>[4x]STPSIVIASAARTAVGSFNGAFANTPAHELGATVISAVLERAGVAAGEVNEVILGQVLPAGEGQNPARQAAMKAGVPQEATAWGMNQLCGSGLRAVALGMQQIATGDASI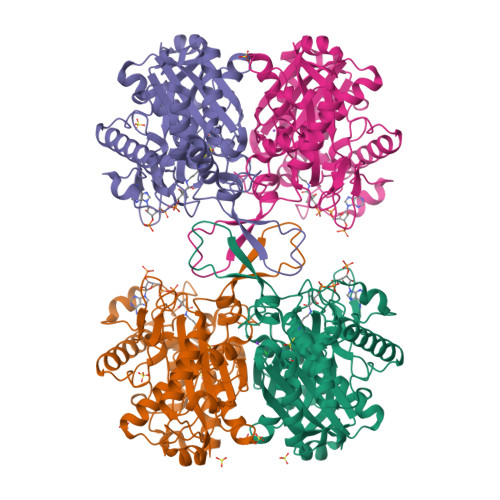IVAGGMESMSMAPHCAHLRGGVKMGDFKMIDTMIKDGLTDAFYGYHMGTTAENVAKQWQLSRDEQDAFAVASQNKAEAAQKDGRFKDEIVPFIVKGRKGDITVDADEYIRHGATLDSMAKLRPAFDKEGTVTAGNASGLNDGAAAALLMSEAEASRRGIQPLGRIVSWATVGVDPKVMGTGPIPASRKALERAGWKIGDLDLVEAAEAFAAQACAVNKDLGWDPSIVNVNGGAIAIGHPIGASGARILNTLLFEMKRRGARKGLATLCIGGGMGVAMCIESL> KK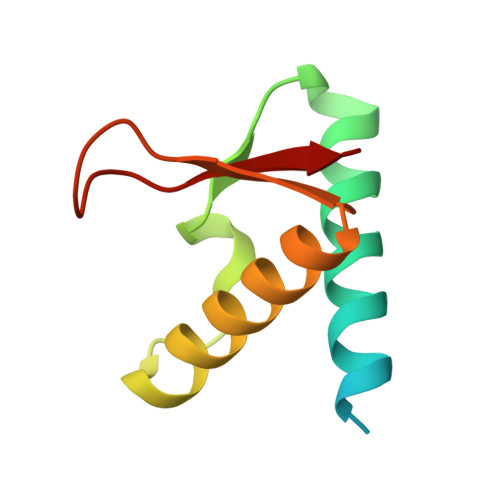VEIDEEIFVIDDFRVDIEKYVEELYKVVKKIYEKTGTPIKFWDLVPDVEPKIIARTFLYLLFLENMGRVEIIQEEPFGEILVVPM>GPMFEARLVQGSILKKVLEALKDLINEACWDISSSGVNLQSMDSSHVSLVQLTLRSEGFDTYRCDRNLAMGVNLTSMSKILKCAGNEDIITLRAEDNADTLALVFEAPNQEKVSDYEMKLMDLDVEQLGIPEQEYSCVVKMPSGEFARICRD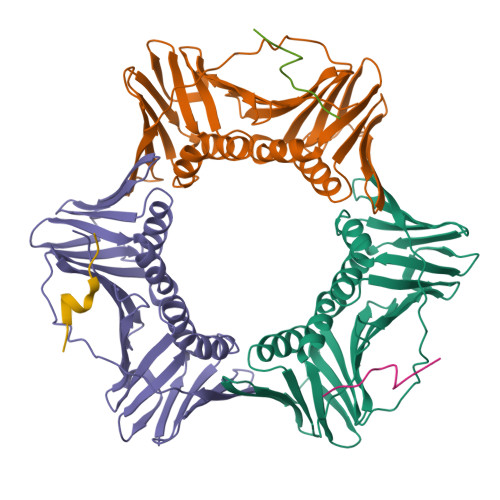LSHIGDAVVISCAKDGVKFSASGELGNGNIKLSQTSNVDKEEEAVTIEMNEPVQLTFALRYLNFFTKATPLSSTVTLSMSADVPLVVEYKIADMGHLKYYLAPKIEDEEGS[3x];>[3x]SSMRKICTYFHRKS> MAHHHHHHMKPDVQQVKAFLLQLQDAICAKLSAVDGKDFVEDSWQREGGGGGRSRVLRNGGIFEQAGVNFSHVHGDAMPASATAHRPELAGRSFEAMGVSLVV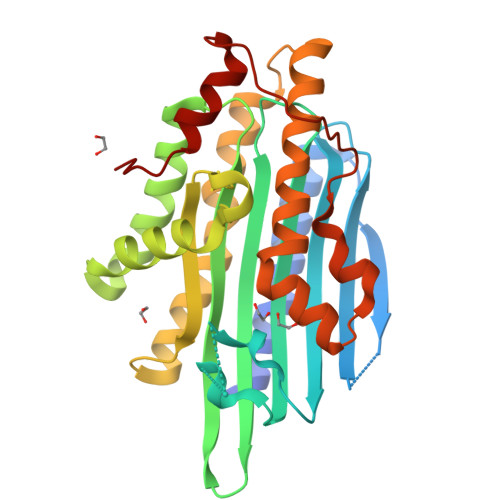HPRNPYVPTSHANVRFFIAEKPGADPVWWFGGGFDLTPYYGFEEDAIHWHRTARDLCLPYGDEVYPRYKKWCDDYFFLKHRNEQRGIGGLFFDDLNTPDFDHCFAFMQAVGNGFTDAYLPIVERRKTTPYGERERDFQLYRRGRYVEFNLVWDRGTLFGLQTGGRTESILMSMPPLVRWEYDYHPQEGSPEAALSEFIKVKEWI N-[(1S)-1-(2-chloro-6-fluorophenyl)ethyl]-5-cyano-1-methyl-1H-pyrrole-2-carboxamide 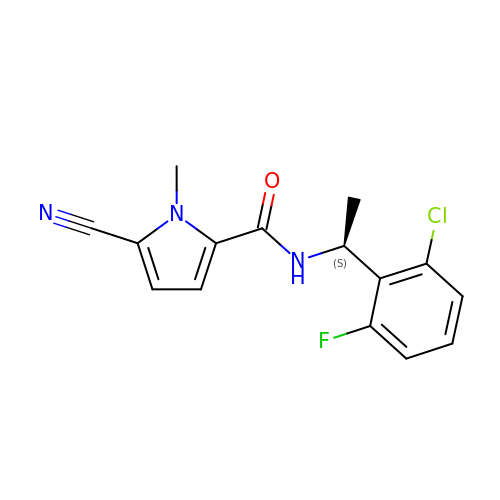| C15 H13 Cl F N3 O | OVRPUVGBRNDNAS-VIFPVBQESA-N Galectins are members of the carbohydrate-binding lectin family with specificity for β-galactosides. The CRD is about 130 amino acids long, and the β-galactoside binding site is conserved among galectins, while differences both in adjacent β-strands and loop regions explain the variation in oligosaccharide binding affinity. Human galectin-7 (hGal-7) is a 15 kDa prototype galectin with a single CRD, monomeric but capable of dimerization in solution. Consequently galectin-7 has shown major roles in cancer development, by helping either in the elimination of certain tumour types or in the growth stimulation of others.

The high resolution structure of hGal-7 in complex with the 2-O-benzylphosphate galactoside inhibitor 6 shows that the synthetic molecule has retained all the conserved interactions involving the galactose moiety, from which it is derived, as well as offering new interactions. The native protein does not show any major conformational change upon binding to the inhibitor 6 with an rmsd of 0.9 Å (all atoms). The phosphate group has a weak hydrogen bonding potential with Arg31, while it is also stabilized by hydrogen-bonded water molecules linked to the same Arg31 and Asn51. The amido group also shows potential interactions with water molecules linked to Lys64 and Trp69, broadening the binding capacity of the ligand to a region not previously involved for galactoside recognition by galectin-7. The phenyl group itself does not seem to be involved in the binding of ligand 6 despite being in close proximity to polar residues His33, Glu122 and Asn35. Interestingly, His33 and Glu122 are not conserved among galectins, thus focusing the ligand interaction towards this position could offer better specificity of inhibition. The anomeric sulfur atom can only weakly interact with a water molecule (3.5 Å) stabilized by Arg31. Interestingly, the benzyl moiety of the O-benzylphosphate 6 is not taking part in the inhibitor binding and faces away from the protein surface. Furthermore, the difference in the crystal packing of the ligand complex structure, highlighted by the different crystallographic cell dimensions compared with the native structure, may be explained by the ligand interaction with a symmetry-related molecule involving residues Arg71 and Arg74 through two potential hydrogen bonds with the phosphate group. This symmetry-related molecule is unique to molecule B of the asymmetric unit and may also explain why only partial electron density was visible for the ligand of molecule A.

>[2x]VPHKSSLPEGIRPGTVLRIRGLVPPNASRFHVNLLCGEEQGSDAALHFNPRLDTSEVVFNSKEQGSWGREERGPGVPFQRGQPFEVLIIASDDGFKAVVGDAQYHHFRHRLPLARVRLVEVGGDVQLDSVRIF> METGNKYIEKRAID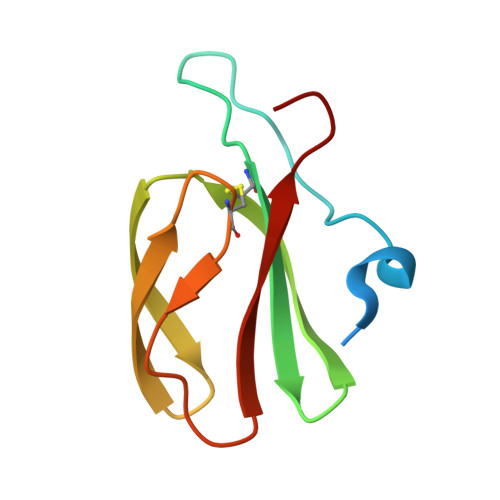LSRERDPNFFDNADIPVPECFWFMFKNNVRQDAGTCYSSWKMDMKVGPNWVHIKSDDNCNLSGDFPPGWIVLGKKRPGF>[2x]MNAAAEAEFNILLATDSYKVTHYKQYPPNTSKVYSYFECREKKTENSKVRKVKYEETVFYGLQYILNKYLKGKVVTKEKIQEAKEVYREHFQDDVFNERGWNYILEKYDGHLPIEVKAVPEGSVIPRGNVLFTVENTDPECYWLTNWIETILVQSWYPITVATNSREQKKILAKYLLETSGNLDGLE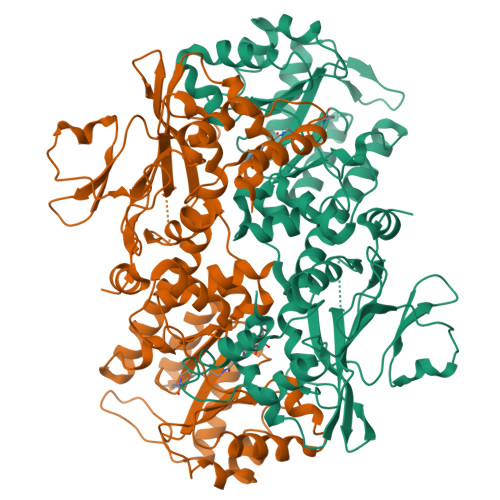YKLHDFGYRGVSSQETAGIGASAHLVNFKGTDTVAGIALIKKYYGTKDPVPGYSVPAAEHSTITAWGKDHEKDAFEHIVTQFSSVPVSVVSDSYDIYNACEKIWGEDLRHLIVSRSTEAPLIIRPDSGNPLDTVLKVLDILGKKFPVSENSKGYKLLPPYLRVIQGDGVDINTLQEIVEGMKQKKWSIENVSFGSGGALLQKLTRDLLNCSFKCSYVVTNGLGVNVFKDPVADPNKRSKKGRLSLHRTPAGTFVTLEEGKGDLEEYGHDLLHTVFKNGKVTKSYSFDEVRKNAQLNMEQDVAPH> MGFIGNSLPMQAVYRVIESAASSKATVFITGESGTGKEVCAEAIHAASPRHDKPFIALNCAAIPKDLIESELFGHVKGAFTGASTERQGAVEMAHNGTLMLDELCEMDLDLQSKLLRFIQTGTYQKVGSSKMSSVDVRFVCATNRNPWEEVQEGRFREDLYYRLHVIPISLPPLRERGGDIIEIAHALLGLMSLEEGKSFSRFSEPVLRLFESYSWPGNVRELQNVIRNIVVLNTDDEVKLEMVPPPILEHHHHHH

Here, we use X-ray crystallography to study LuxO, the central quorum sensing regulator in Vibrio cholerae and related bacteria. LuxO belongs to the subfamily of AAA+ ATPases known as bacterial enhancer-binding proteins (bEBPs). In LuxO, as in NtrC proteins, the phosphorylation of an aspartate located within the R-domain activates the C domain for ATP hydrolysis and the opening/activation of σ54-dependent promoters. Here, we present crystal structures and in vitro and in vivo functional studies of LuxO that together reveal what is, to our knowledge, an entirely novel mechanism of AAA+ protein regulation, in which a regulatory segment of the protein prevents substrate ATP binding and hydrolysis by occupying a portion of the enzyme active site.

The most potent of these, with an EC50 in V. cholerae of 4.1 μM, was a tert-butyl analog previously called compound 12 and here renamed AzaU. To characterize the mechanism of AzaU inhibition of LuxO, we crystallized V. angustum LuxO-C in the absence of ligands (apo), in the presence of ATP, and in the presence of AzaU. AzaU bound in the LuxO active site, with its modified uracil ring occupying the same region as the adenine ring of the ATP substrate, indicating that AzaU functions as a competitive inhibitor. Indeed, consistent with this structural inference, ATPase assays using LuxO-C showed that AzaU inhibition is enhanced at lower ATP concentrations, as expected for a competitive inhibitor. Strikingly, AzaU binds the LuxO active site in a manner that mimics the R-C linker, with both AzaU and the R-C linker forming H-bonds with Arg 316 and Gln 363. All three protein structures are highly similar (rms deviation < 0.5 Å). Rather than forming closed rings, V. angustum LuxO monomers in the crystals form continuous helical arrays with six subunits per turn. We also observed the same helical arrays of LuxO monomers in crystal structures of the V. angustum C domain alone (LuxO-C), either as the apo-protein, with ATP bound, or with the inhibitor AzaU bound (discussed below). Our crystal structures do not reveal any substantial conformational changes associated with AzaU, CV-133, or ATP binding, possibly because of constraints imposed by the crystal lattice. In particular, the conformation of the GAFTGA loop, implicated in σ54 binding, is unaffected by either inhibitors or ATP, adopting in all cases a conformation similar to that of ADP-bound NtrC1. Alternatively, extending the idea that AzaU recapitulates some of the key interactions that stabilize the R-C linker in the ATPase active site, it may prove possible to engineer potent and selective second-generation inhibitors that capture even more of these interactions.>PFLELDTNLPANRVPAGLEKRLCAAAASILGKPADRVNVTVRPGLAMALSGSTEPCAQLSISSIGVVGTAEDNRSHSAHFFEFLTKELALGQDRILIRFFPLESWQIGKIGTVMTFL[3x]

pmcThe human macrophage migration inhibitory factor (MIF) superfamily, comprised of MIF and D-dopachrome tautomerase (DDT, also called MIF-2), is broadly and constitutively expressed with involvement in proinflammatory and host antimicrobial responses. MIF and MIF-2 are highly similar in structure, with monomeric units of 114 and 117 amino acids, respectively, that form homotrimers. An evolutionarily conserved proline at the N terminus acts as the catalytic base for a tautomerization reaction of unknown biological significance in both proteins. The same site in MIF-2 is Phe100 and is also evolutionarily conserved among all MIF-2 proteins, suggesting this site plays an important role in both proteins.

Crystal structures of the wt proteins show that the side chains of wt-MIF and wt-MIF-2 are similarly oriented, suggesting that the intermolecular forces stabilizing both relays between the enzymatic and allosteric sites are consistent. A major difference between MIF-2 and MIF is the replacement of the solvent channel of MIF with a large solvent cavity in MIF-2. Because it is primarily the addition of a large side chain at Phe2 that pushes the channel outward, the solvent cavity of wt-MIF-2 does not contain any more waters than wt-MIF (41 versus 42) despite the expansion in the upper cavity. This is also likely because the bottom of the MIF-2 channel is largely blocked by Arg42, causing this cavity to appear truncated relative to MIF, which instead has a valine at the same position. Another interesting feature is the dense region of waters in a horizontal layer just above the Arg42 side chain of MIF-2. This is due to an increase in charged, hydrophilic residues in this area of MIF-2 (Arg42, Glu4), while MIF has the hydrophobic Leu and Ile residues at these positions. The N-terminal nitrogen of F100A and S62A differs from that of wt-MIF-2 by 1.7 Å and 0.8 Å, respectively. These differences are influenced by tartrate in the wt-MIF-2 active site with two hydrogen bonds from the Pro1 nitrogen to the tartrate carboxylate (2.9 Å) and carbonyl (2.7 Å) oxygens that stabilize its position. wt-MIF-2 is the only protein in this study that has tartrate in its crystallization conditions. To understand the loss of ∼60% of enzymatic activity in F100A relative to wt-MIF-2, the superimposed wt-MIF-2 and F100A structures were examined using tartrate (from crystallization conditions of wt-MIF-2) in the electropositive active site as a guide. Seven wt-MIF-2 residues with atoms within 4 Å of the tartrate were compared with the same residues of F100A. We next assessed the crystallographic water networks for wt-MIF-2 and three variants and found wt-MIF-2 to have the densest network of water molecules.> HGFVDNATIGGQFYQFYQPYQDPFMGSPPDRISRKIPGNGPVEDVTSLAIQCNADSAPAKLHASA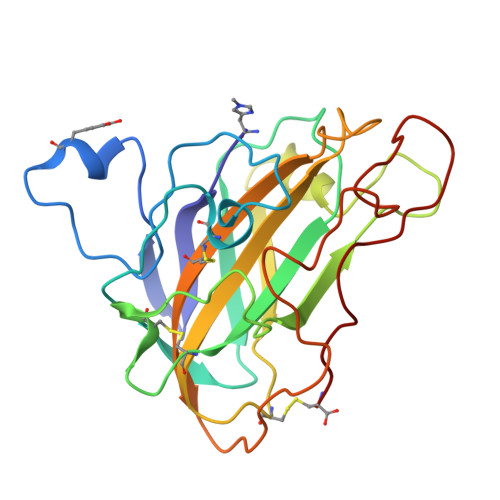AAGSTVTLRWTIWPDSHVGPVITYMARCPDTGCQDWTPSASDKVWFKIKEGGREGTSNVWAATPLMTAPANYEYAIPSCLKPGYYLVRHEIIALHSAYSYPGAQFYPGCHQLQVTGSGTKTPSSGLVSFPGAYKSTDPGVTYDAYQAATYTIPGPAVFTC>[4x]MLRSSLLPFSYLYEKIINFRNTLYDKGFLKIKKLPVPVISVGNLSVGGSGKTSFVMYLADLLKDKRVCILSRGYKRKSKGTLIVSEYGNLKVSWEEAGDEPYLMAKLLPHVSVVASEDRYKGGLLALEKLSPEVFILDDGFQHRKLHRDLNILLLKKKDLKDRLLPAGNLREPLKEIRRADALVLTYQEVEPFEFFTGKPTF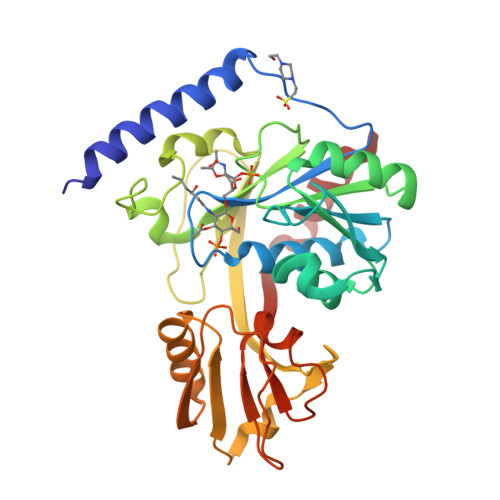KMFREFCCLLNSDFEEVPFDILKEREVIAFSGLGDNGQFRKVLKNLGIKVKEFMSFPDHYDYSDFTPEEGEIYLTTPKDLIKLQGYENVFALNFKVKLEREEKLKKLIYRIFY> GAMGSNVIFEDEEKSKMLARLLKSSHPEDLRAANKLIKEMVQEDQKRMEKISKRVNAI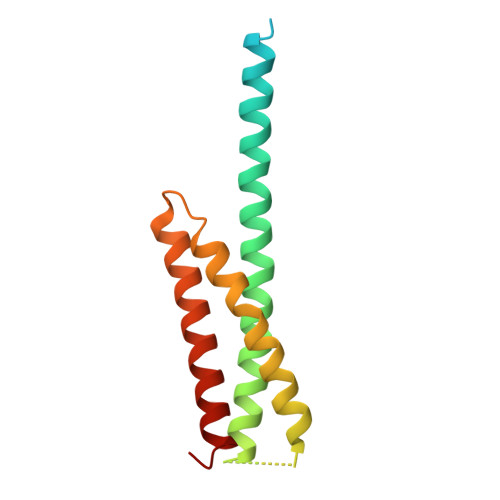EEVNNNVKLLTEMVMSHSQGGAAAGSSEDLMKELYQRCERMRPTLFRLASDTEDNDEALAEILQANDNLTQVINLYKQLVRGEE The protein belongs to the αβ-hydrolase superfamily and is related to the bacterial hormone-sensitive lipase (HSL) family of enzymes as concluded from structural similarity searches with DALI. Here, we present the crystal structure of the carboxylesterase LpEst1 from L. plantarum WCFS1 at 2.05 Å resolution. This structure revealed that although LpEst1 belongs to the bacterial HSL family of enzymes, as otherwise expected from its sequence, it represents a novel topological variant due to the presence of large and specific structural features that decorate a canonical αβhydrolase core. Additionally, the esterase forms dimers in the crystal and in solution through an association mode not observed yet in any other αβhydrolase enzyme. The structural homology found with enzymes from the bacterial HSL family permitted the straightforward identification of the catalytic machinery of LpEst1 as a classical catalytic triad with Ser174 as the nucleophile, His313 as the general base that deprotonates the serine hydroxyl and Asp283 as the residue that increases the pKa of the histidine imidazole ring.

The four independent molecules of the LpEst1 asymmetric unit are arranged in two identical dimers, consisting of the pairs A–C and B–D. The independent molecules are almost perfectly superimposable with an overall rmsd value of 0.42 Å as determined with PDBeFOLD. According to the analyses with PISA and PIC servers, the subunits within each dimer generate an interface area of 1130 Å2 and interact via 19 hydrogen bonds and 24 hydrophobic interactions. In summary, taken as a whole, these results demonstrate that LpEst1 is a dimer despite the relative low overall interaction energies calculated at the interface and further suggest, that the apolar interactions are the main driving force for dimerization.

>[4x]GGSHHHHHHGENLYFQGMPTINSIQTTVNGVVKIVKPFNNDIAGEQFDPHVLQTLTAFKQPAILENDLAALRSGSLTPAIADPVGDAVTVQSRNITALNRTVSVEWLTPQNVINHTVLVYFHGGAFYGGVPGNNTVLLKLVAAKSHCEILNVDYSLAPEAPAPAGILDGLAIFQYLEQRDAETMITVAGDSAGANVIMAATNLNQQLGSNRINQQLLLYPVTAPNADHAGPLWDLAAFPIIDSQRAILTNYHDLFRQLDSIMTDYYVPENFDSHSPLISPLHQENFTMTPPTTIMVGEFDPFRPQAWAYAQRLAAADTATTFIQYQGLNHAFAPLVDQYWQSQDVAQVMAAALI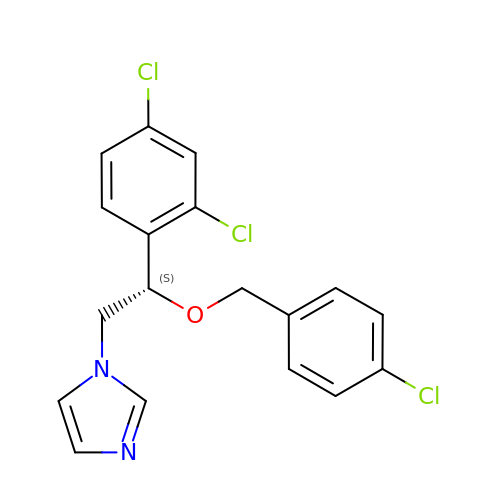1-[(2S)-2-[(4-CHLOROBENZYL)OXY]-2-(2,4-DICHLOROPHENYL)ETHYL]-1H-IMIDAZOLE | C18 H15 Cl3 N2 O | LEZWWPYKPKIXLL-GOSISDBHSA-N> ALRGTVTDFSGFDGEADAEVLRKAMEGLGTDEDSILNLLTARSNAQRQQIAEEFETLFGRDLVNDMKSELTGKFEKLIVALMKPSRLYDAYELKHALKGAGTDEKVLTEIIASRTPEELRAIKQAYEEEYGSNLEDDVVGDTS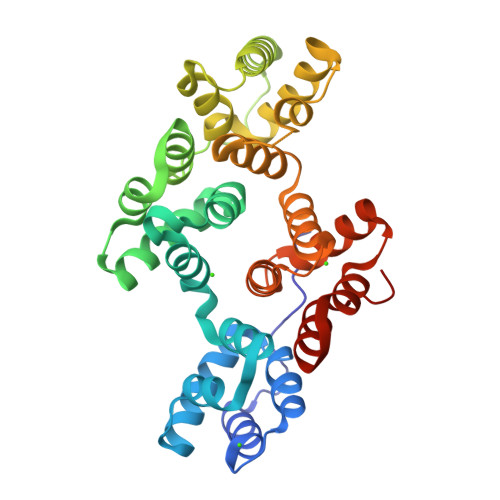GYYQEMLVVLLQANRDPDTAIDDAQVELDAQALFQAGELKWGTDEEEFITILGTRSVSHLRRVFDKYMTISGFQIEETIDRETSGNLENLLLAVVKSIRSIPAYLAETLYYAMKGAGTDDHTLIRVIVSRSEIDLFNIRKEFRKNFATSLYSMIKGDTSGDYKKALLLLSGGEDD> GAASMEFPFDVDALFPERITVLDQHLRPPARRPGTTTPARVDLQQQ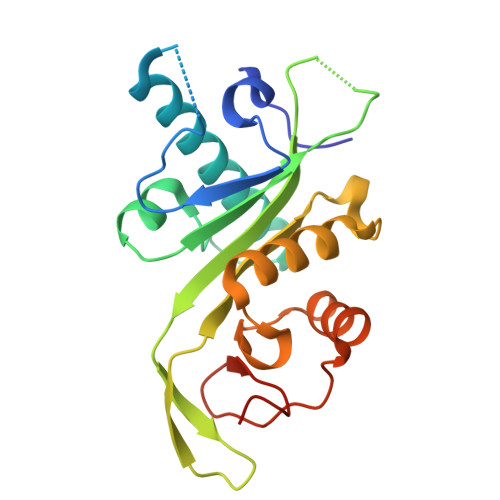IMTIIDELGKASAKAANLSAPITSASRMQSNRHVVYILKDSSARPAGKGAIIGFIKVGYKKLFVLDDREAHNEVEPLCILDFYIHESVQRHGHGRELFQYMLQKERVEPHQLAIDRPSQKLLKFLNKHYNLETTVPQVNNFVIFEGFFAHQHRP> GAKPYEKVRIYRMDGSYRSVELKHGNNTTVQQIMEGMRLSQETQQYFTIWICSENLSLQLKPYHKPLQHVRDWPEILAELTNLDPQRETPQLFLRRDVRLPLEVEKQIEDPLAILILFDEARYNLLKGFYTAPDAKLITLASLLLQIV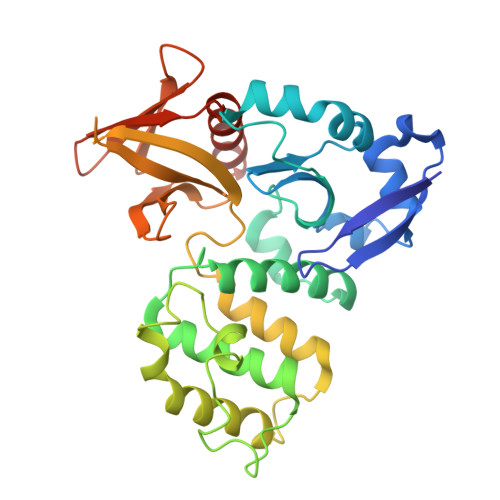YGNYESKKHKQGFLNEENLKSIVPVTKLKSKAPHWTNRILHEYKNLSTSEGVSKEMHHLQRMFLQNCWEIPTYGAAFFTGQIFTKASPSNHKVIPVYVGVNIKGLHLLNMETKALLISLKYGCFMWQLGDTDTCFQIHSMENKMSFIVHTKQAGLVVKLLMKLNGQLMPTERNS> GSSGSSGDCVQLNQYTLKDEIGKGSYGVVKLAYNENDNTYYAMKVLSKKKLIRQAGFPRR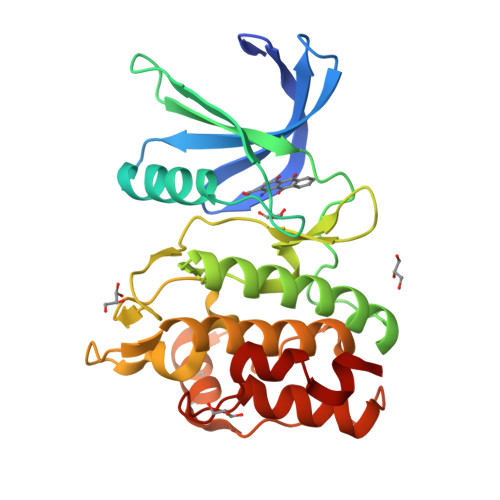PPPRGTRPAPGGCIQPRGPIEQVYQEIAILKKLDHPNVVKLVEVLDDPNEDHLYMVFELVNQGPVMEVPTLKPLSEDQARFYFQDLIKGIEYLHYQKIIHRDIKPSNLLVGEDGHIKIADFGVSNEFKGSDALLSNTVGTPAFMAPESLSETRKIFSGKALDVWAMGVTLYCFVFGQCPFMDERIMCLHSKIKSQALEFPDQPDIAEDLKDLITRMLDKNPESRIVVPEIKLHPWVTR2-{[(naphthalen-2-yl)sulfonyl]amino}-5-[(2-phenylethyl)sulfanyl]benzoic 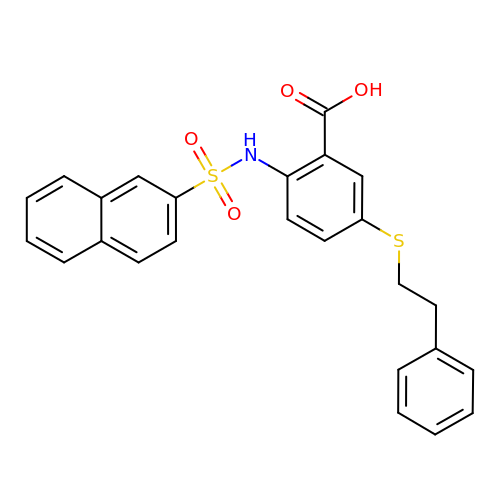acid | C25 H21 N O4 S2 | NSEKHDVVZNMXDE-UHFFFAOYSA-N>[2x]HHHHHHDDDDKRTLPGEGTQVHPRAPLLQILKVAGAQEEVFTVKEVMHYLGQYIMMKQLYDKQRQHIVHCHDDPLG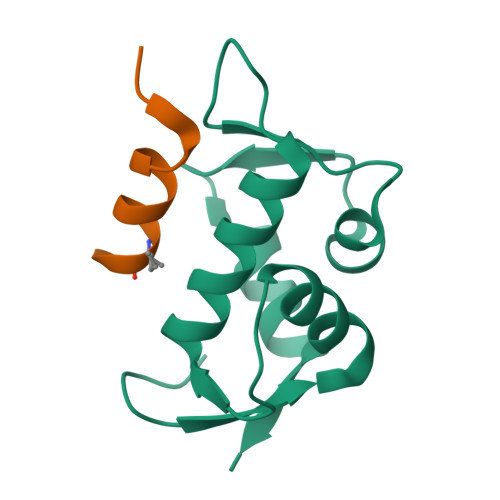ELLEVGSFSVKNPSPLYEMLKRNLVIL;>LSQETFXDLWKLLLENX[2x]> MGYYDIDDVLADGTEFPCKFQYDIPGLGYLENNPGRPITKNTKLSLPLWLARILAIVGGDEALVDEEPVPFVELLPPDMFSTKVMNAI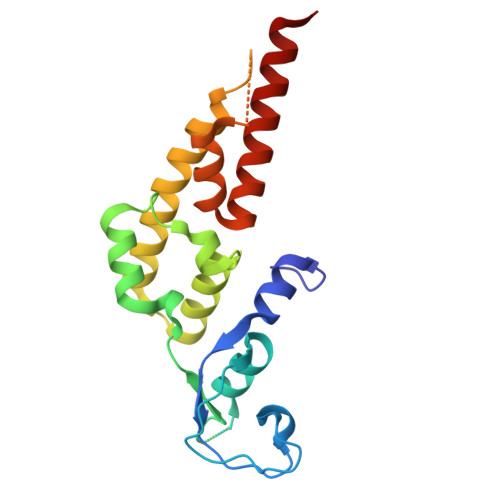KTDPVALDLHSINSHFFSLAIKWIMLFSEKELANVVSELLLQRAQELNHHASSLSIDLNADSTGKNSANTNIATSTFLLKLEEMEKEIYKKSHESYKDTKRWMFKK> EFAITSCPNNETVWETPIGVKYTLCPGSDYQNGGASLQTVRDIQSSLECAKICDSDARCNRAVYDNVNKACDVKNSTNPMQWAADDRFETIRLTNDLPEGAFISTCSFNETSYRVPETNAEYRICPDTDYTGVNAKVVEGVTTIQACAELCSNTQDCRKSVFDHINNACAIKAAEPATSIFWVQDKQFSTIRLPENIDPAVKGKWGDLIRLPVIPVAAYIVPSYPEPSRLLFFSSWSNDAFSGASGMTQFGDYDFATGAISQRTVTNTHHDMFCPGISQLEDGRILIQGGSDADTVSIYDPATNEFTRGPNMTLARGYQTSCTLSNGKVFTIGGAYSGERVGKNGE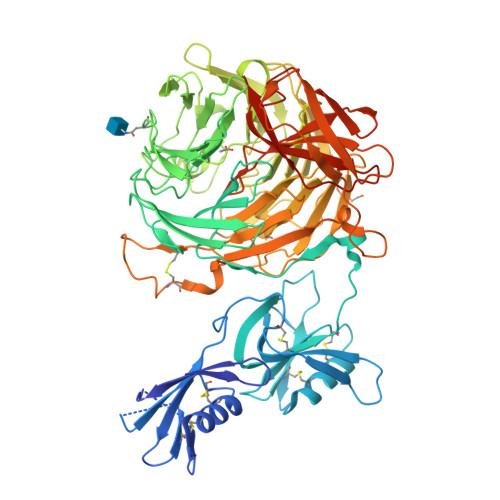VYDPVANAWTYLPGADFRPMLTNDHEGIWREDNHAWLFGWKNGSIFQAGPSKDQHWYGIQGNGTVAKAATRDDDDAMCGVWVMYDAVAGKIFSAGGSPDYTDSPATQRAHITTIGEPNTPAEVERVADMGFPRGFANAVVLPDGQVLVTGGQRMSLVFTNTDGILVAELFNPETREWKQMAPMAVPRNYHSVSILLPDATVFSGGGGMCWVQNVGDSTAGCDKTVDHSDGEIFEPPYLFNEDGSRAARPVISAISADPIKAGATLTFTVEGVEGQGTAALIRLGSVTHSVNSDQRRVPLNVTVSGNEYSATLPDDYGILLPGYYYLFVSTPQGTPSIAKTVHVILGLEQKLISEEDLNSAVDHHHHHH>[4x]DDLPDSIDWRENGAVVPV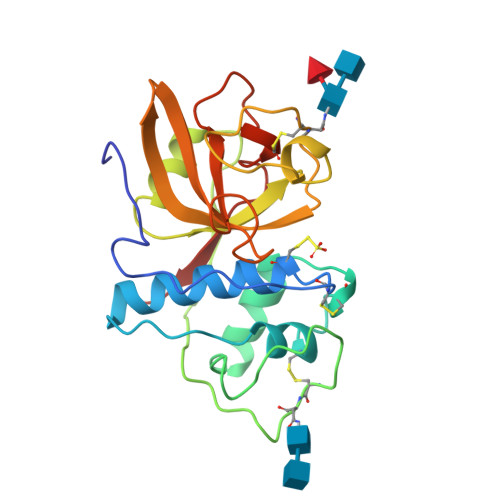KNQGGCGSCWAFSTVAAVEGINQIVTGDLISLSEQQLVDCTTANHGCRGGWMNPAFQFIVNNGGINSEETYPYRGQDGICNSTVNAPVVSIDSYENVPSHNEQSLQKAVANQPVSVTMDAAGRDFQLYRSGIFTGSCNISANHALTVVGYGTENDKDFWIVKNSWGKNWGESGYIRAERNIENPDGKCGITRFASYPVKKGTN> SNAGGGVTFCGGEPLLHPEFLIDILKRCGQQGIHRAVDTTLLARKETVDEVMRNCELLLIDLKSMDSTVHQTFCDVPNELILKNIRRVAEADFPYYIRIPLIEGVNADEK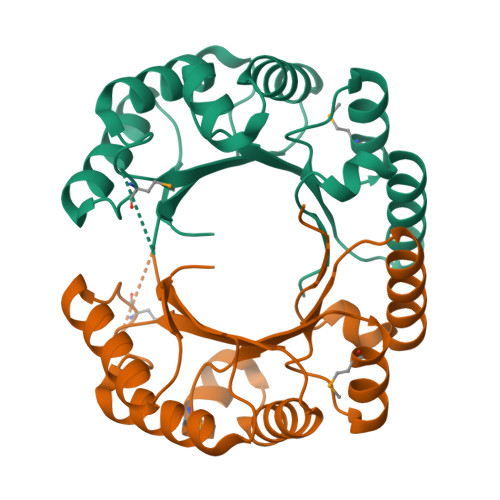NIKLSAEFLASLPRHPEIINLLPYHDIGKGKHAKLGSIYNPKGYKMQTPSEEVQQQCIQILTDYGLKATIGG> MKKLEKKLSAEPINFDSFFSEKAMLMKASEVRELLKLVETSDVISLAGGLPAPETFPVETIKKIAVEVLEEHADKALQYGTTKGFTPLRLALARWMEKRYDIPMSKVEIMTVAGSQQALDLIGRVFLNPGDPIVVEAPTYLAAIQAFK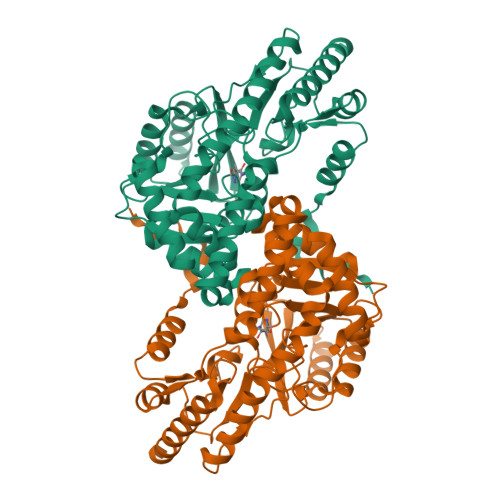YYDPEFISIPLDDKGMRVDLLEEKLEELRKQGKRVKIVYTVSTFQNPAGVTMSVDRRKKLLELANEYDFLIVEDGPYSELRYSGEPTPPIKHFDDYGRVIYLGTFSKILAPGFRIGWVAAHPHLIRKMEIAKQSIDLCTNTFGQAIAWKYVENGYLDEHIPKIIEFYKPRRDAMLEALEEYMPEGVEWTKPEGGMFVRVTLPEGIDTKLMMERAVAKGVAYVPGEAFFVHRDKKNTMRLNFTYVPEETIREGVRRLAETIKEEMKRVKG>SSQIRQNYSTDVEAAVNSLVNLYLQASYTYLSLGFYFDRDDVALEGVSHFFRELAEEKREGYERLLKMQNQRGGRALFQDIKKPAEDEWGKTPDAMKAAMALEKKLNQALLDLHALGSARTDPHLCDFLETHFLDEEVKLIKKMGDHLTNLHRLGGPEAGLGEYLFERLTLKH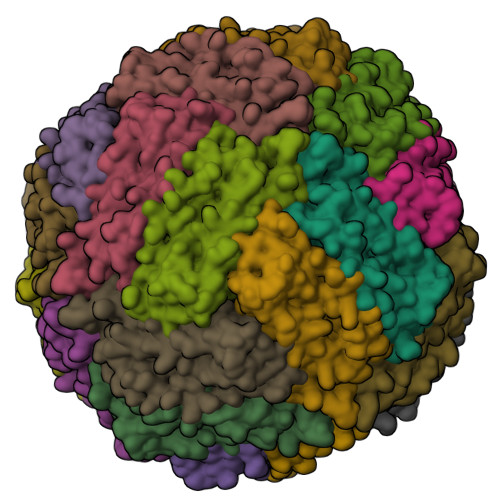D[24x]>[2x]SNAMKFDDSKPIYKQIVHYIHTEIVTGTYEAGDKLLSVRELATKLEVNPTTIQRAYAELEETEIIYTV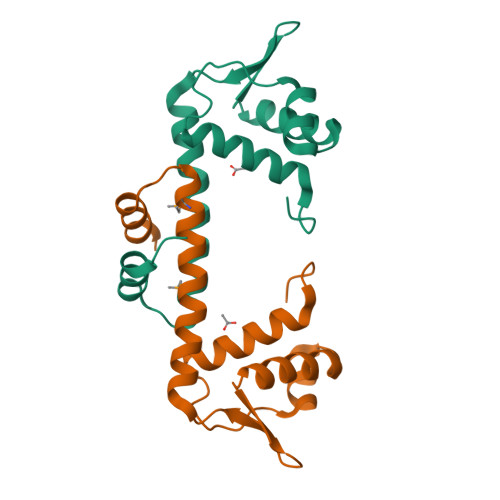RGTGKYLTEDKRRIEQLENDIAKQLTENFISEMSKLGINKEKIIAWVKKVEEVEVNVSGK> MGKSTLTFLIAGCLALPGFARAADAADPALVKRGEYLATAGDCMACHTVKGGKPYAGGLGMPVPMLGKIYTSNITPDPDTGIGKWTFEDFERAVRHGVSKNGDNLYPAMPYVSYAKITDDDVRALYAYFMHGVEPVKQAPPKNEIPALLSMRWPLKIWNWLFLKDGPYQPKPSQSAEWNRGAYLVQGLAHCSTCHTPRGIAMQEKSLDETGGSFLAGSVLAGWDGYNITSDPNAGIGSWTQQQLVQYLRTGSV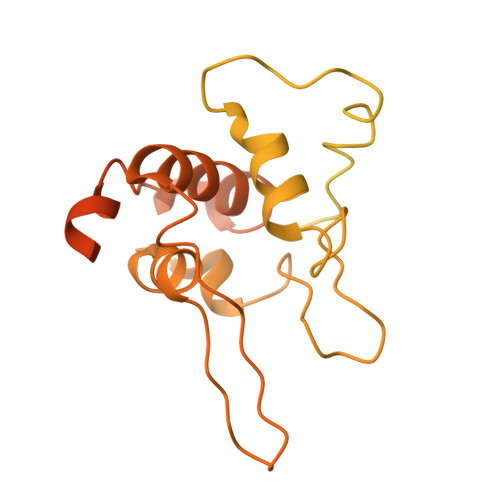PGVAQAAGPMAEAVEHSFSKMTEADIGAIATYVRTVPAVADSNAKQPRSSWGKPAEDGLKLRGVALASSGIDPARLYLGNCATCHQMQGKGTPDGYYPSLFHNSTVGASNPSNLVQVILNGVQRKIGSEDIGMPAFRYDLNDAQIAALTNYVTAQFGNPAAKVTEQDVAKLRSGGPVPLLVRVRPLMLPGAVVVVLIALLGVAFWWRRRQRTPLANPPQGKAGHHHHHH>[5x]MDQITRILEKLNQQRSGETTVTLADFMPMSLAEIRSQNTGRLSREEAQLLHRAAQKEKQNNILYTARMLTRANPLLKKEMNTARYYGATPYGYDDIIPPRAEKFVAPGAVSSMFSPAGYLTELYREARGLHPKDSDRNLDKRRQDLAKLVLSQDNLDNEISALSLANEQLETALMAQTGKTDKNKYYETLATSRRSGVTPYNAPFEGIHNALAQRNFVLPDNILSNPAKFAILAAYDAGISPKLYNILTEDTESLTGSDLENSLKRNFPKVKIKDLMTLDALANYYELPADDIQALIAAEITGRLPTPDVYNDDNKLVIPAINTGGKITFSELAKTQSDEKQADYIDLIPQGGNQFLVNFSVKKTKKDATHFSIGYNKSFNNLADKNGFVPLAGEHYSIPVTLDAKILEKKTKIGITRKKPEPASDENHYTSATFTIHPNAEPGIWLLRLNKTLRLAKVSGMTPHETQHALIHVRNDSSEYELRRFTETLLYRKRYGIDTETALMLCNAGISRISYDGQLSHFDRLFNNPPLNGVTYTLGGDDILMEPDAGDPRREVLKRAFRVDNTGLWQLLVITNRENKSKTIENKTEKLRGLLFVRLLADVHNLTVAQLDALLQISPYNSMNVYALDGKTRQKMLSFLSRITQWLNTQNITVEQLMLLLDKISPAAPTKEMQVLLDLLRNGGIDKTNTKTLYTTMAPVITAAMQLDITESGEALLRWLDNNHPAGILTTSEARKLIIKKGQTAGDKEKLAAWCQALAQRVLVIRTFTLSNAELQTLSQGAPAGTITELYNISDFHNLINRCGEQAGTVLDALQSGTLTVKILAQALNLSEEVITQALTLAGQKPELTTWAQLAVLPPRLDLADTLHITPKDITTLLTVSENVRPFYTDLSALAGLLQAGLNEQQTKQLQNQSEPRRNEALSGEYRSLVMNNPVADRDDIWRNLLVDGKVSAEITTTLLADAIAGIQLYINRTIAGDEPGADSDALERQFFKDWDACNKRYSTWAGVSQLVYYPENFVDPTLRTGQTGMMNTMLEQLSQSELNKDTLENGFRQYLTAFEQVADLKVVSGYHDTVNINQGNTWFIGTSQTEPKKYYWRKADHSKCQNGRFAANAWSDWKEITCAVNPYGDMVRPVIFHSRLYLLWIEKQVQKDNTGKDTASFTLKLTHVKYDGSWASPFSYDITEKNISGWKKTGLYCAASQEDNSLLIAWYQIEKETQPNSFGLHIQPDMSCKKEPNIAGILATVTHQLDTETTVRVNTLLNRISSFEFTLEKQEGNKEIDLVISHGDYTVKTENSISALILNPTAYINITPYKLFSDIPDFYREKYITHLNSHSGTVYAPESKKMEPANNAISDKVNACAVYTYNNKPPKKHISLSIGKNYPLITPLELVGRKLESFFIKHKETSALYYTYGDATDDRLTLEEDKYTISTGEKKLGTLSLGKMIAQVKTISSDDISMEIELNSTKFETITGSDVGLRPPLYPTVSRETLAFPFGKLSITIPAGADINNLDCTIKVRFKNTDVLAATTTYKLVIKKTDPVQKVISLYTTPDGAQYMEWDGYRTRLNTLFTRQLIERANNGIDAILSPETQYLPEPKPGQGTYVTLILKPYDKNTHGTNRAFTIYYSNDATGSGKFPVYSGSLSVTDNTEVKLFIPLIKPGKNAVSQSAGAQQDTLYLNATYQ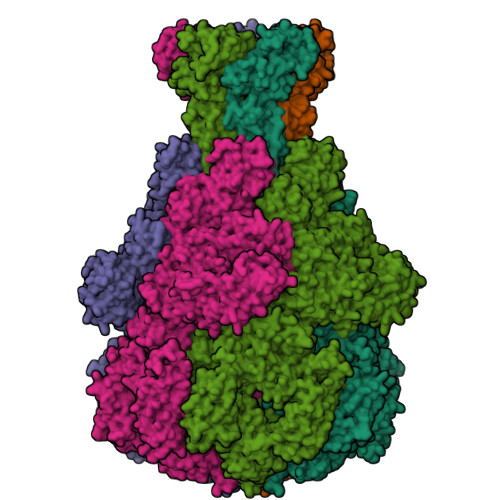KEATKQILLFRTDNNPEGWTLDKSVNNGTFAGLAENGVTGLLQSGEPMDFSGANALYFWELFYYTPMMVATRLLQEQNFTEANRWLSYIWQPAASGAGDWRVRPLKEDTSWNADPLDSVDPDAVAQNDPMHYKVSTLMKLLDLLIARGDKAYRMQERDTLNEAKMWYMQALGLLGDKPVSIFSNGWENPSLSNAADKTQAKQFHDEISRIRSGGLLPDVRTANTLTGLFRPQQNEKLLGYWQMLEMRLFNLRNNLSIDGQPLSLPVFAAPADPAALLSAAAAASGGSKPLPSADIPAMRFPQALDSARSLTGQLMQFGSTLLGLIERRDAEAMSELLQNQAGELMLSSLRMQEQALTELDAEKKILEQSRAGAQSRVDSYRALYDENVSAEEKRTMDLYLSSAILSTSIGVLDMAAAAADMAPNIFGVAVGGSRWGGIPKAIGAGMSLAASATKITADNISQSEAWRRRRQEWEIQKNNAESEIRQIDAQLEALAVRRTATEMQREHMEIQQAQTQAQLEFLQRKFSNKALYSWLRGRLASIYYRFYDLTAARCMMAEKAYAWQTNDTATRYIKSGAWQSNNAGLMAGESLLLNLAEMEQAWLKRDSRSLEVTRTVSLAAVYRTDNVTLAEGIADLLKGNGSGNIPASTGLSMTADNQLHAAFNLKALNIKDDYPEALGTTRRIKQISVTLPALVEPYQDMRAIFRYGGNSLPAGCKAIALSHGINDDGLFRLDFNDGRWLPFEGIPVDDDNSLTLSFPDATGEKQKPLLLSLTDIIIHIRYTIC> MLFGRLTERAQRVLAHAQEEAIRLNHSNIGTEHLLLGLMKEPEGIAAKVLESFNITEDKVIEEVEKLIGHGQDHVGTLHYTPRAKKVIELSMDEARKLHHNFVGTEHILLGLIRENEGVAARVFANLDLNITKARAQVVKALGNPEMSNKNAQASKSNNTPTLDSLARDLTVIAKDGTLDPVIGRDKEITRVIEVLSRRTKNNPVLIGEPGVGK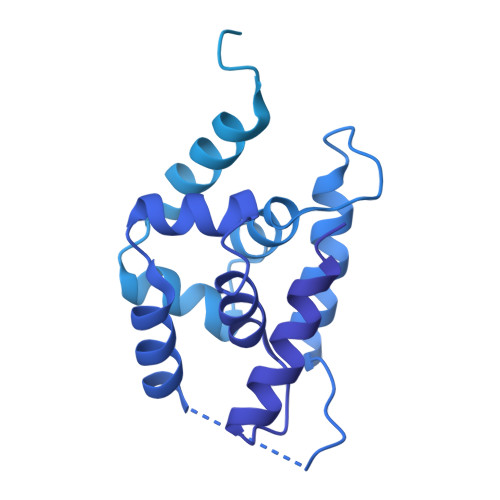TAIAEGLAQAIVNNEVPETLKDKRVMSLDMGTVVAGTKYRGEFEERLKKVMEEIQQAGNVILFIDELHTLVGAGGAEGAIDASNILKPALARGELQCIGATTLDEYRKNIEKDAALERRFQPVQVDEPSVVDTVAILKGLRDRYEAHHRINISDEAIEAAVKLSNRYVSDRFLPDKAIDLIDEASSKVRLKSHTTPNNLKEIEQEIEKVKNEKDAAVHAQEFENAANLRDKQTKLEKQYEEAKNEWKNAQNGMSTSLSEEDIAEVIAGWTGIPLTKINETESEKLLSLEDTLHERVIGQKDAVNSISKAVRRARAGLKDPKRPIGSFIFLGPTGVGKTELARALAESMFGDDDAMIRVDMSEFMEKHAVSRLVGAPPGYVGHDDGGQLTEKVRRKPYSVILFDEIEKAHPDVFNILLQVLDDGHLTDTKGRTVDFRNTIIIMTSNVGAQELQDQRFAGFGGSSDGQDYETIRKTMLKELKNSFRPEFLNRVDDIIVFHKLTKEELKEIVTMMVNKLTNRLSEQNINIIVTDKAKDKIAEEGYDPEYGARPLIRAIQKTIEDNLSELILDGNQIEGKKVTVDHDGKEFKYDIAEQTSETKTPSQA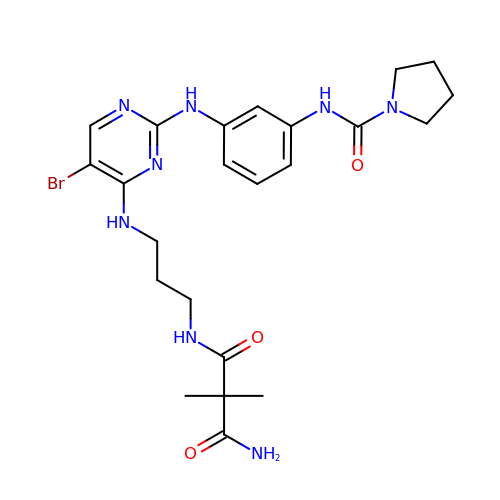N-(3-{[5-BROMO-2-({3-[(PYRROLIDIN-1-YLCARBONYL)AMINO]PHENYL}AMINO)PYRIMIDIN-4-YL]AMINO}PROPYL)-2,2-DIMETHYLMALONAMIDE | C23 H31 Br N8 O3 | ZNSULAZTNWFKEW-UHFFFAOYSA-N> VRAPALSNPRGRIHCRLVAKKELSRDVRLFRFSLPSPDQVLGLPIGKHIFVCATIEGKLCMRAYTPTSMVDEIGHFDLLVKVYFKNEHPKFPNGGLMTQYLDSLPVGSYIDVKGPLGHVEYTGRGSFVINGKQRNARRLAMICGGSGITPMYQIIQAVLRDQPEDHTEMHLVYANRTEDDILLRDELDRWAAEYPDRLKVWYVIDQVKRPEEGWKYSVGFVTEAVLREHVPEGGDDTLALASGPPPMIQFAISPNLEK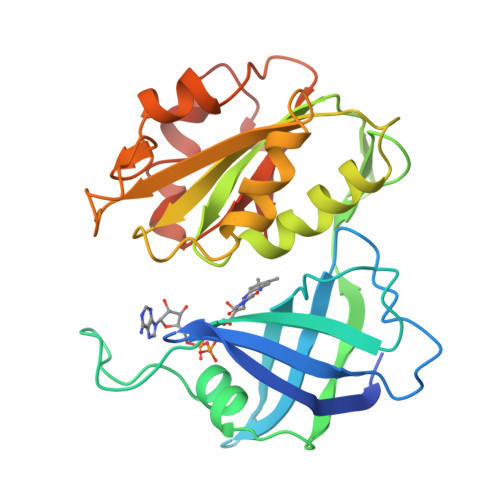MKYDMANSFVVF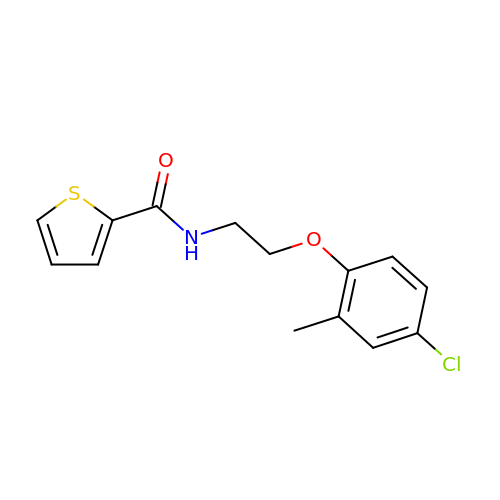N-[2-(4-chloro-2-methylphenoxy)ethyl]thiophene-2-carboxamide | C14 H14 Cl N O2 S | RULQUKFOBAPKKR-UHFFFAOYSA-N>[2x]MKADAVKIADGVYWVGVLDWDIRMYHGYTLNGTTYNAYLVFGDDKVALIDNTYPGTSAQMWGRIKDACEKEGREFKIDVIVQNHVEKDHSGALPEIHKKFPEAPIYCTEVAVEGLVKHFPSLKGAPFKVVKSLESIDLGGKTLTFLEAPLLHW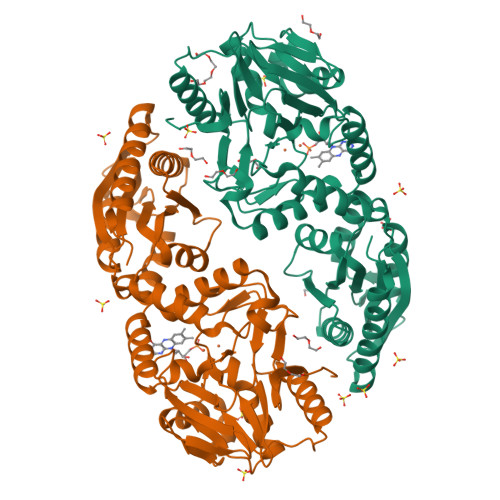PDSMFTLYAEEGILFSNDAFGQHLCFTQRFDHEIPENILMDANQKFYANLITPLSKLVLKKFKEVIELGLLEKIKMIAPSHGQIWTDPMKVIGAYQDFATGKCKDKVTIVYDTMHGSTQKMAHAFAEGIMSEGVDVKMYFLHNDERSEIVKDILDSKAFLLGAPTIYDEPFPSVGDLIYYLKGLKFNRTGLKRLALAFGSMGGNGGGTKVLAEKLKECGFEVLDEYELYYVPTEDELEKCYNMGKRLAVKVKEMKTE>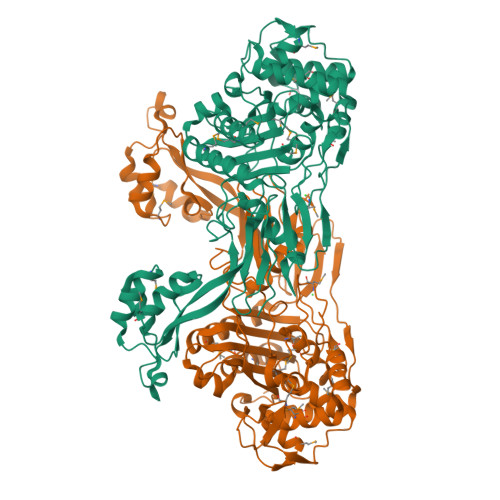SNATGHSNGQDLVMKANEKYLVKNAQQPERGKIYDRNGKVLAEDVERYKLVAVIDKKASANSKKPRHVVDKKETAKKLSTVINMKPEEIEKRLSQKKAFQIEFGRKGTNLTYQDKLKIEKMNLPGISLLPETERFYPNGNFASHLIGRAQKNPDTGELKGALGVEKIFDSYLSGSKGSLRYIHDIWGYIAPNTKKEKQPKRGDDVHLTIDSNIQVFVEEALDGMVERYQPKDLFAVVMDAKTGEILAYSQRPTFNPETGKDFGKKWANDLYQNTYEPGSTFKSYGLAAAIQEGAFDPDKKYKSGHRDIMGSRISDWNRVGWGEIPMSLGFTYSSNTLMMHLQDLVGADKMKSWYERFGFGKSTKGMFDGEAPGQIGWSNELQQKTSSFGQSTTVTPVQMLQAQSAFFNDGNMLKPWFVNSVENPVSKRQFYKGQKQIAGKPITKDTAEKVEKQLDLVVNSKKSHAANYRIDGYEVEGKTGTAQVAAPNGGGYVKGPNPYFVSFMGDAPKKNPKVIVYAGMSLAQKNDQEAYELGVSKAFKPIMENTLKYLNVGKSKDDTSNAEYSKVPDVEGQ[2x]>[6x]FMQDFEDIQKDIEQLDIKCAHEQMNIQKQYDEKKKPLFEKRDEIIQKIPGFWANTLRKHPALSDIVP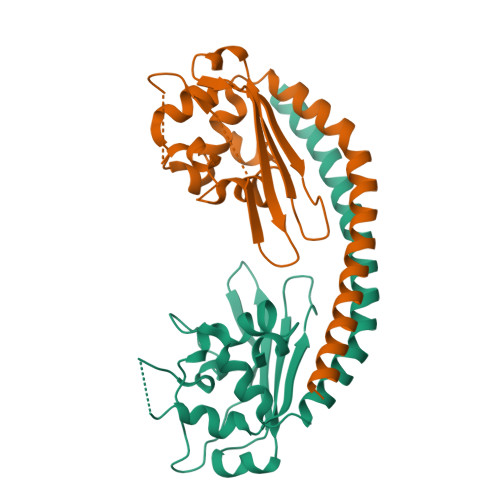EDIDILNHLVKLDLKDNMDNNGSYKITFIFGEKAKEFMEPLTLVKHVTFDNNQEKVVECTRIKWKEGKNPIAAVTHNRSDLDNEIPKWSIFEWFTTDELQDKPDVGELIRREIWHNPLSYYLGLEE> GGAGGGGAAAUUCUAUCUGGUGAUAGACGGGAACUCUAAAUUCCUUGAAAUGCCUCGCCGCAUUGGGUUCGAUUCCCUUCCCCUCCGCCA

A search of metagenomic sequences revealed uniquely structured tRNAs (allo-tRNAs) containing recognition elements that resembled tRNASec but with a 12 bp acceptor domain (acceptor and T-stem combined) for proper recognition by EF-Tu. Specifically, tRNAUTu1 was found to be a serine isoacceptor with a 9/3 (acceptor/T-stem bp) structure that allowed EF-Tu driven Sec incorporation. Here, we investigated the suitability of an allo-tRNA, tRNAUTu1, for translation by E. coli ribosomes, and demonstrate the importance of global tRNA structure for efficient translation. tRNAUTu1 is used for site-specific insertion of Sec by harnessing EF-Tu to avoid constraints on natural Sec translation. Implementing cryo-EM, we visualized tRNAUTu1 in complex with the E. coli ribosome to pinpoint the structural feature in tRNAUTu1 hindering translation.

We hypothesized that disrupting the A45:C8 interaction might destabilize the central loop, which could lead to higher flexibility of the variable loop, resulting in lower rates of ribosome splitting and improved processivity of ribosomes after suppression. We made a C8A mutation to reduce the likelihood that a base pair would form with A45 (tRNAUTu1A). Data processing and particle sorting resulted with two maps, each with either A site tRNAUTu1A or P site tRNAUTu1A alone. The structure of tRNAUTu1A revealed this disrupted interaction without altering the position of the variable arm in the A site. Instead, the absence of the C8:A45 mismatch base pair in the core of tRNAUTu1A created flexibility in the variable arm such that it could move cooperatively with the ASF in transition from the A to the P site. A single nucleotide mutation (C8A) removed the translational roadblock, increasing protein expression to match that of a natural suppressor tRNA (tRNAsupD).>[2x]MHHHHHHSTATNPLDLDVCAREPIHIPGLIQPYGVLLVIDPADGRIVQASTTAADLLGVPMAALLGMPYTQVLTLPEAQPFAVDDQPQHLMHAEVRFPQRATPPASAWVAAWHLYPQQWLVEMEPRDARLLDVTLREAMPLLRSVERDPGIAEAAVRVAKGLRSLIGFDRVMIYRFDEEWNGDIIAEARKPELEAYLGQHYPASDIPAQARALYLRNRVRQIADVGYQPSPIQPTVHPQLGTPVDLSDVSLRSVSPVHLEYLANMGVTATLVASIVVNDALWGLISCHHYSPHFTNHAMRDVTDAVARTLAGRIGALQAVARARLESVLLTVREKLITDFNDAEHMTVELLDDMAPDLMDVVDADGVAIFHGNDISRHGTTPDVAALRRIRDHIESEHHEALREDAVGALHVDAIGEVFPELADLAPLAAGFIFVPLMPQSRSALLWTRREQIQQIKWAGNPQLAKLEDIPNSRLSPRK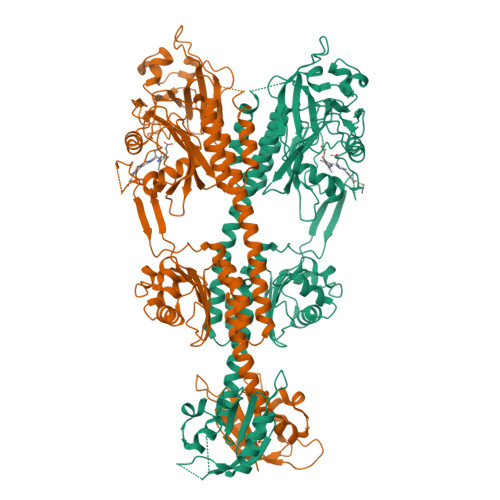SFDLWQQTVRGRARRWSPLHLESARSLRVLIELMERKRFQQDFTLLEASLSRLRDGVAIIERGTANAAHRLLFVNTAFADVCGSDVAELIGRELQTLYASDAPRANVELLQDALRNGRAAYVTLPLQVSDGAPVYRQFHLEPLPSPSGVTAHWLLQLRDPE> MSQSKKETPLASLLFDDVEKINHDQDYWFQLRGDNPNVLIDAATPLFGLSLRVRTLTECDNIEQIYRQTIEEIKAIEIELTEQGYEHAILMAYRYILCAFLDESVMGTEWGA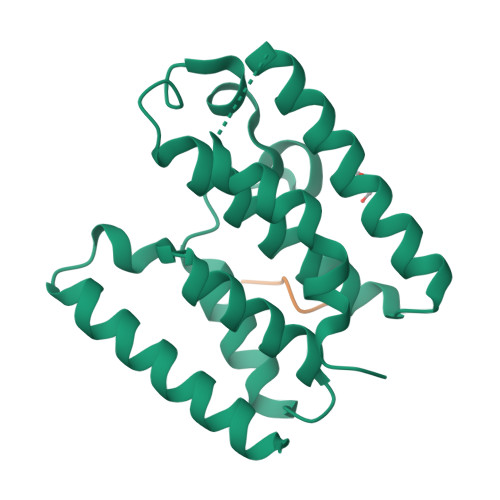SSLWAEHSMLSRFHNETWGGEKVFTILSRLEGEPHRYQALLAFIYHCLILGFEGKYRVMEGGQAEREKVISRLHQLLSSLEESEPQDLTRPTDHVVRAKYTLSRQMPVWSVFAGFIVLWVGLFLGYSYVLHSKSSDVLNQLNQIL;> DLTRP>[4x]SNAQSPQKAGTKRTDAPPVMEQVGYGETIGMLVVPKWYGVTNNN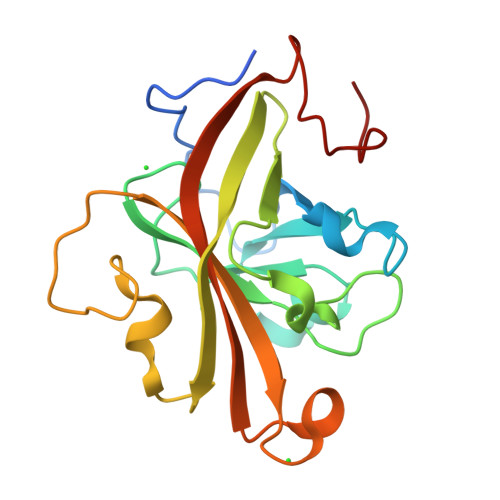MPIMEGTGSDVLDQAAAGHYTNTQQLGEVGNFAIAGHRRTYGNSFRRIDLLQEGDEIIVSTAKTWYVFKVTGHELVKPEQVEVIAPVPNQPDAQPTDRYITLTTCHGSTAGEFGNDLRWIVHAKFAYWMDRSEGRPESVLNDPGVN> AVSSSRGGI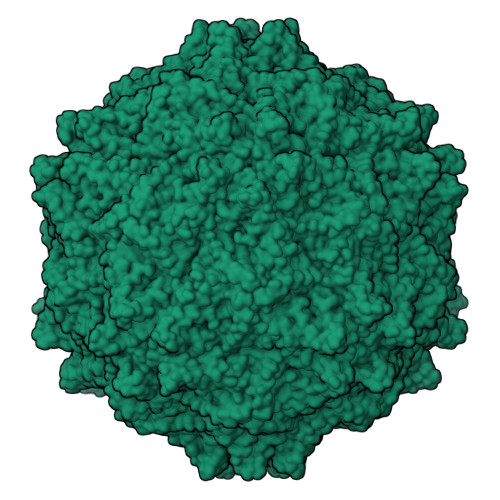TVLTHSELSAEIGVTDSIVVSSELVMPYTVGTWLRGVAANWSKYSWLSVRYTYIPSCPSSTAGSIHMGFQYDMADTVPVSVNQLSNLRGYVSGQVWSGSAGLCFINGTRCSDTSTAISTTLDVSKLGKKWYPYKTSADYATAVGVDVNIATPLVPARLVIALLDGSSSTAVAAGRIYCTYTIQMIEPTASALNN>GCCGCCGC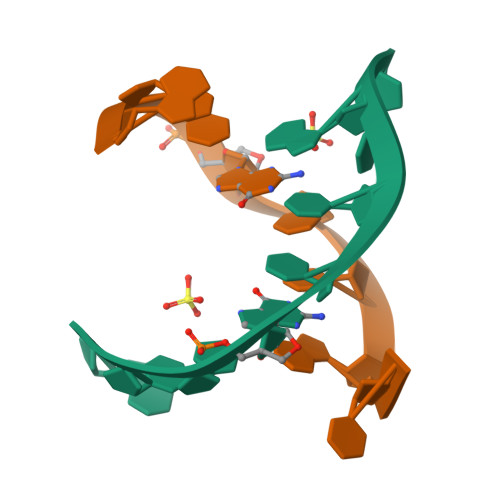[3x]>SEGSDAPNFVLEDTNGKRIELSDLKGKGV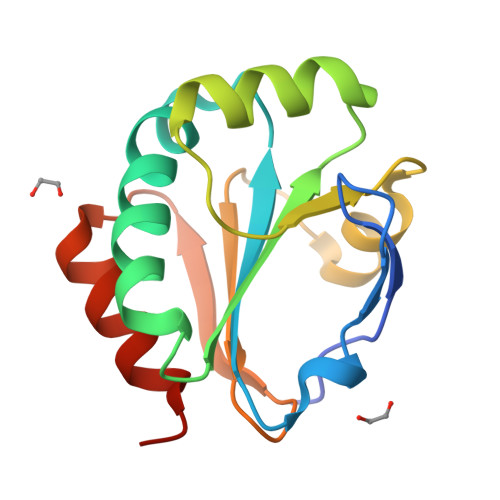FLNFWGTWAEPCKKEFPYMANQYKHFKSQGVEIVAVNVGESKIAVHNFMKSYGVNFPVVLDTDRQVLDAYDVSPLPTTFLINPEGKVVKVVTGTMTESMIHDYMNLIKPGETSG[2x]> GSHMASPNGQTKPLPALKLALEYIVPCMNKHGICVVDDFLGKETGQQIGDEVRALHDTGKFTDGQLVSQKSDSSKDIRGDKITWIEGKEPGCETIGLLMSSMDDLIRHCNGKLGSYKIKERTKAMVACYPGNGTGYVRHVDNPNGDGRCVTCIYYLNKDWDAKVSGGILRIFPEGKAQFADIEPKFDRLL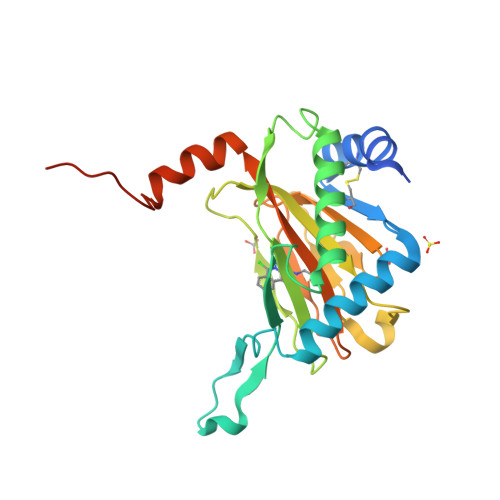FFWSDRRNPHEVQPAYATRYAITVWYFDADERARAKVKYLTGEKGVRVELNKPSDSVGKDVF> SMRQREQQLLEFLDRLTSLLESKGKVKTKKLQSMLGSLRPAHLGPCSDGHYQ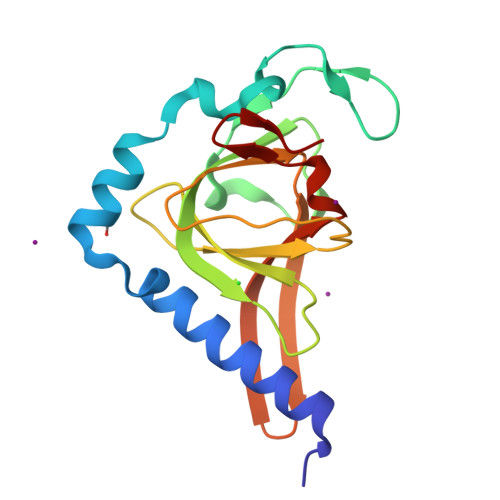SASGQKVTLELKPLSTLQPGVNSGAVILGKVVFSLTTEEKVPFTFGLVDSDGPCYAVMVYNIVQSWGVLIGDSVAIPEPNLRLHRIQHKGKDYSFSSVRVETPLLLVVNGKPQG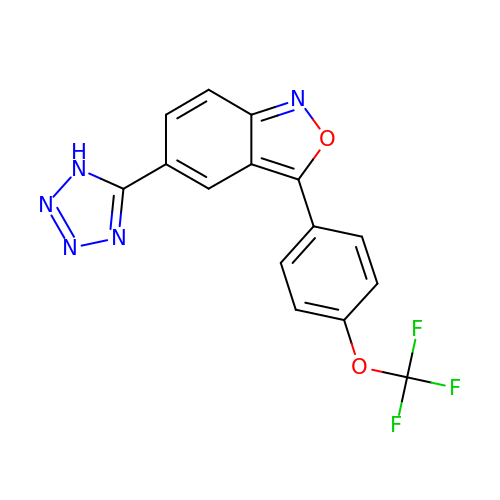(5P)-5-(1H-tetrazol-5-yl)-3-[4-(trifluoromethoxy)phenyl]-2,1-benzoxazole | C15 H8 F3 N5 O2 | OPRMMWAPDMWRES-UHFFFAOYSA-N N-(tert-butoxycarbonyl)-3-methyl-L-valyl-(4R)-4-[(7-chloro-4-methoxyisoquinolin-1-yl)oxy]-N-{(1R,2S)-1-[(cyclopropylsulfonyl)carbamoyl]-2-ethenylcyclopropyl}-L-prolinamide 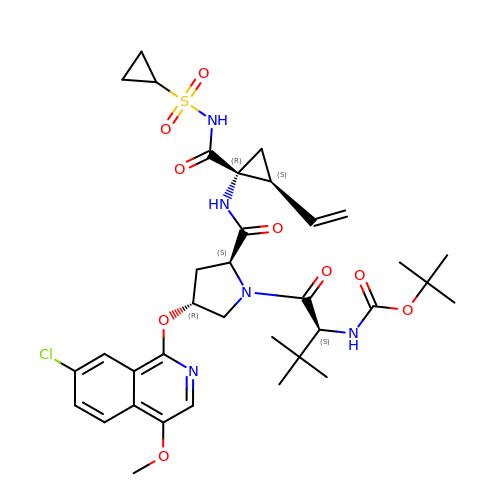| C35 H46 Cl N5 O9 S | XRWSZZJLZRKHHD-WVWIJVSJSA-N> GSSHHHHHHSSGLVPRGSMSTSWSDRLQNAADMPANMDKHALKKYRREAYHRVFVNRSLAMEKIKCFGFNMDYTLAVYKSPEYESLGFELTVERLVSIGYPQELLSFAYDSTFPTRGLVFDTLYGNLLKVDAYGNLLVCAHGFNFIRGPETREQYPNKFIQRDDTERFYILNTLFNLPETYLLACLVDFFTNCPRYTSCETGFKDGDLFMSYRSMFQDVRDAVDWVHYKGSLKEKTVENLEKYVVKDGKLPLLLSRMKEVGKVFLATNSDYKYTDKIMTYLFDFPHGPKPGSSHRPWQSYFDLILVDARK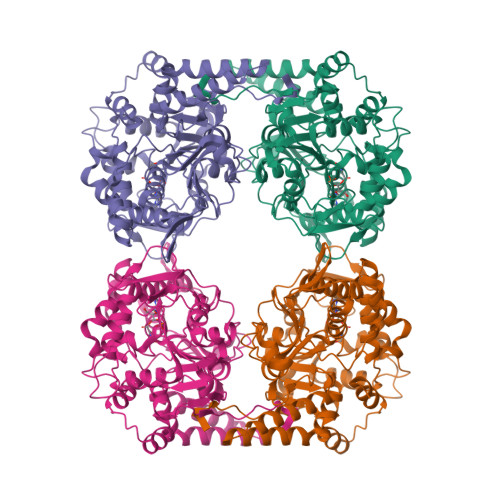PLFFGEGTVLRQVDTKTGKLKIGTYTGPLQHGIVYSGGSSDTICDLLGAKGKDILYIGDHIFGDILKSKKRQGWQTFLVIPELAQELHVWTDKSSLFEELQSLDIFLAELYKHLDSSSNERPDISSIQRRIKKVTHDMDMCYGMMGSLFRSGSRQTLFASQVMRYADLYAASFINLLYYPFSYLFRAAHVLMPHESTVEHTHVDINEMESPLATRNRTSVDFKDTDYKRHQLTRSISEIKPPNL In the CU pathway, a dedicated chaperone facilitates the folding of pilus subunits in the periplasm and an integral outer membrane (OM) protein termed the usher provides the assembly platform and secretion channel for the pilus fiber. Periplasmic chaperone–subunit complexes are then recruited to the OM usher (PapC for P pili, FimD for type 1 pili) for subunit assembly into pili and secretion of the pilus fiber to the cell surface. Ushers contain five domains: a central 24-stranded ß-barrel domain that inserts into the OM to form the secretion channel, an internal plug domain that forms the channel gate, a periplasmic N-terminal domain (NTD) that functions in subunit recruitment, and two tandem periplasmic C-terminal domains (CTD1 and CTD2) that function in pilus assembly and secretion. Using cryo-electron microscopy (EM), we determined structures of the activated PapC usher in the process of secreting two- and three-subunit P pilus assembly intermediates.

To generate a three-subunit intermediate, we replaced the PapK NTE with the NTE from PapE (PapKE-NTE) and deleted papE, resulting in a ∆E P pilus tip fiber composed of PapK bound to PapF bound to PapG. For the three-subunit ∆E dataset, starting with 537,038 particles, after 2D and 3D classifications, we derived one 3D map, named Conformer I at 7.6 Å. The ∆E cryo-EM structure (Conformer I) represents a P pilus assembly intermediate consisting of the PapC usher, PapD chaperone, and three polymerized pilus subunits: the PapG adhesin, with its pilin domain translocating through the PapC β-barrel channel and its lectin domain exposed on the extracellular side; and PapF and PapK, which are located on the periplasmic side of the usher. PapK is bound to the PapD chaperone via DSC, and PapK is also linked (by its engineered PapE NTE) to PapF via DSE. PapF in turn is engaged in DSE with the pilin domain of PapG. In the Conformer I ∆E structure, the PapD chaperone and associated PapK subunit are held on the periplasmic side of the PapC usher by the N-terminal tail region of the usher NTD. Notably, PapC CTD2 is not resolved in the ∆E structure, indicating that this usher domain is released from the bound chaperone-tip complex and flexible. Therefore, Conformer I likely represents the stage just after a newly recruited chaperone–subunit complex (PapDK), still bound at the usher NTD, has undergone DSE with the previously recruited chaperone–subunit complex (PapDF) bound at the usher CTDs. Comparison with the ∆E Conformer I shows that as the third subunit is polymerized from below, PapG moves upward (outward) by 41 Å while rotating by 85°, which is equivalent to approximately 2° rotation per 1 Å advance. Notably, as the PapG lectin domain emerges from the usher chamber, it bends back by 60° toward the pilin domain such that the two lobes of PapG are now nearly orthogonal to each other.

> VEFNTDVLDAADKKNIDFTRFSEAGYVLPGQYLLDVIVNGQSISPASLQISFVEPQSSGDKAEKKLPQACLTSDMVRLMGLTAESLDKVVYWHDGQCADFHGLPGVDIRPDTGAGVLRINMPQARLEYSDATWLPPSRWDDGIPGLMLDYNLNGTVSRNYQGGDSHQFSYNGTVGGNLGPWRLRADYQGSQEQSRYNGEKTTNRNFTWSRFYLFRAIPRWRANLTLGENNINSDIFRSWSYTGASLESDDRMLPPRLRGYAPQITGIAETNARVVVSQQGRVLYDSMVPAGPFSIQDLDSSVRGRLDVEVIEQNGRKKTFQVDTASVPYLTRPGQVRYKLVSGRSRGYGHETEGPVFATGEASWGLSNQWSLYGGAVLAGDYNALAAGAGWDLGVPGTLSADITQSVARIEGERTFQGKSWRLSYSKRFDNADADITFAGYRFSERNYMTMEQYLNARYRNDYSSREKEMYTVTLNKNVADWNTSFNLQYSRQTYWDIRKTDYYTVSVNRYFNVFGLQGVAVGLSASRSKYLGRDNDSAYLRISVPLGTGTASYSGSMSNDRYVNMAGYTDTFNDGLDSYSLNAGLNSGGGLTSQRQINAYYSHRSPLANLSANIASLQKGYTSFGVSASGGATITGKDAALHAGGMSGGTRLLVDTDGVGGVPVDGGQVVTNRWGTGVVTDISSYYRNTTSVDLKRLPDDVEATRSVVESALTEGAIGYRKFSVLKGKRLFAILRLADGSQPPFGASVTSEKGRELGMVADEGLAWLSGVTPGETLSVNWDGKIQCQVNVPETAISDQQLLLPCTPQK;> AVSLDRTRAVFDGSEKSMTLDISNDNKQLPYLAQAWIENENQEKIITGPVIATPPVQRLEPGAKSMVRLSTTPDISKLPQDRESLFYFNLREIPPRSEKANVLQIALQTKIKLFYRPAAIKTRPNEVWQDQLILNKVSGGYRIENPTPYYVTVIGLGGSEKQAEEGEFETVMLSPRSEQTVKSANYNTPYLSYINDYGGRPVLSFICNGSRCSVKKEK;> MIRLSLFISLLLTSVTVLADVQINIRGHVYIPPCTINNGQNIVVDFGNINPEHVDNSRGEVTKTISISCPYKSGSLWIKVTGNTMGGGQNNVLATNITHFGIALYQGKGMSTPLTLGNGSGNGYRVTAGLDTARSTFTFTSVPFRNGSGILNGGDFRTTASMSMIYN;> MKKWFPALLFSLCVSGESSAWNNIVFYSLGDVNSYQGGNVVITQRPQFITSWRPGIATVTWNQCNGPGFADGFWAYYREYIAWVVFPKKVMTQNGYPLFIEVHNKGSWSEENTGDNDSYFFLKGYKWDERAFDAGNLCQKPGETTRLTEKFDDIIFKVALPADLPLGDYSVKIPYTSGMQRHFASYLGARFKIPYNVAKTLPRENEMLFLFKNIGGCRPSAQSLEIKHGDLSINSANNHYAAQTLSVSCDVPANIRFMLLRNTTPTYSHGKKFSVGLGHGWDSIVSVNGVDTGETTMRWYKAGTQNLTIGSRLYGESSKIQPGVLSGSATLLMILP;> MIKSTGALLLFAALSAGQAIASDVAFRGNLLDRPCHVSGDSLNKHVVFKTRASRDFWYPPGRSPTESFVIRLENCHATAVGKIVTLTFKGTEEAALPGHLKVTGVNAGRLGIALLDTDGSSLLKPGTSHNKGQGEKVTGNSLELPFGAYVVATPEALRTKSVVPGDYEATATFELTYR>[5x]HHHHHHMALQLAAHSDARSGPVGSNGGQFWSFRPVRPLNKIVLSFSGSPDQTLNLISITFSSNPTDIITVGGVGPEPLTYTETVNIDGDIIEISGMIANYKGYNVIRSIKFTTNKKEYGPYGANAGTPFNIKIPDGNKIVGFFGNSGWYVDAIGAYYTAK

Structural and functional analysis identified IPO as a member of the JRL family but with a different tetrameric association. The monomeric IPO from residues 1 to 154 shows a typical β-prism fold found in the JRL family, with 12 β-sheets (β3-β14) and 2 additional short, extended, N-terminal β-strands (β1-β2). Four IPO protomers form a compact tetrameric association by swapping their extended N termini from residues 1 to 10. Thus, the wound-inducible protein IPO from sweet potato has versatile carbohydrate binding properties and might play a role in plant defense.

The apo IPO showed an orthorhombic space group of I222. A reasonable volume of the unit cell (Vm) for the Matthew coefficient was estimated at 2.19 Å3/Da and 44% solvent content by 8 IPO molecules. However, only 5 IPO molecules in an asymmetric unit could be built after molecular replacement. We obtained a higher Matthew coefficient with 3.51 Å3/Da and 65% solvent content. In the packing diagram for apo IPO, we observed a tetrameric association with an additional monomer in an asymmetric unit. The additional monomer could form a tetrameric association with the other 3 neighboring molecules, which were generated by symmetric operations (-X, Y, -Z), (X, -Y, -Z), and (-X-1, -Y, Z). So 4 IPO molecules could form a tetramer.The genus Enterovirus comprises numerous human pathogens, including rhinoviruses, polioviruses, echoviruses and other human-infecting viruses like EV-A71 and EV-B93. Coxsackie virus 3C protease, like other enteroviral proteases, is a cysteine protease with a characteristic specificity for glutamine in the P1 position of its substrates. Thus, for this target, fragments binding to the S1 pocket are biomimetics of the glutamine side chain, while the active-site nucleophile is the thiolate of cysteine 147 (Cys-147).

Compounds 12, 14 and 20 were incubated with EV-B93 3C protease. The protein complex with 14 gave well-diffracting crystals, which showed the presence of additional electron density in the active site corresponding to the molecular structure of the inhibitor. As described by our docking studies, exclusively the electrophilic C-2 of 14 was attacked and covalently linked to the nucleophilic Cys-147, forming a stable tetrahedral Michael addition product. As a result, 14 is inserted between the solvent-exposed β-strand E2 and the loop formed by Thr-142, Arg-143, and Ala-144 and occupies the S1 and S1′ sub-pockets of the protein. Other than the reference inhibitor AG-7404, which is attacked at C-3 (see asterisk), the C-1 carbonyl oxygen of the ethyl amide in 14 is oriented towards the oxyanion hole and forms a hydrogen-bonding network with the backbone amides of Cys-147, Gln-146 and Gly-145. The N-ethyl group points into the S1′-pocket. The pyrazolone ring of 14 is sandwiched in the S1 pocket by π−π interactions with the peptide bonds between Arg-143—Ala-144 on one side and the Gly-164—Asn-165 on the other side. The pyrazol-5-amide NH interacts with Arg-143, Gly-164, and a water molecule that mediates a hydrogen bond to His-161. The cycloheptane shows only weak electron density indicating the flexible orientation of this part of the molecule at the protein surface, a van der Waals interaction is observed between the ring C4 atom and the side-chain Cβ atom of Ala-144. The modified warhead structure seems to favour binding through an additional interaction with the oxyanion hole and with the π-stacking of the pyrazolone.

>MKGPAFEFAVAMMKRNASTVKTEYGEFTMLGIYDRWAVLPRHAKPGPTILMNDQEVGVLDAKELVDKDGTNLELTLLKLNRNEKFRDIRGFLAREEVEVNEAVLAINTSKFPNMYIPVGQVTDYGFLNLGGTPTKRMLVYNFPTRAGQCGGVLMSTGKVLGIHVGGNGHQGFSAALLRHYFNEEQHHHHHH[2x]> METVVGLTAIAVALLIGLGALGTA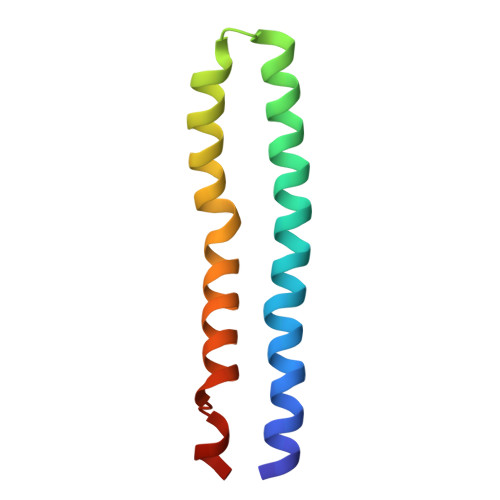IGFGLLGGKFLEGAARQPEMVPMLQVKMFIVAGLLDAVTMIGVGIALFFTFANPFVGQIAG> SSSNYCNQMMKSRNLTKDRCKPVNTFVHESLADVQAVCSQKNVACKNGQTNCYQSYSTMSITDCRETGSSKYPNCAYKTTQANKHIIVACEGNPYVPVHFDASV;> K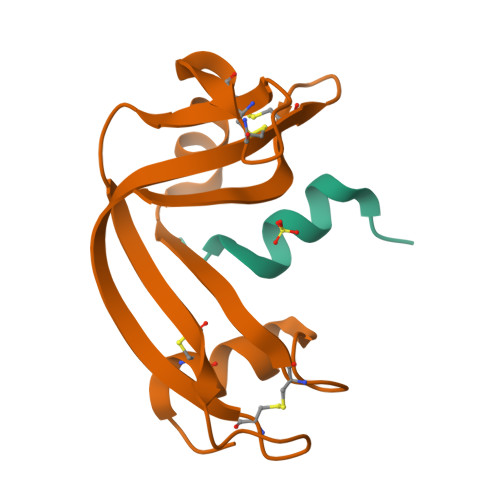ETAAAKFERQHIDSX> MNHKVHHHHHHIEGRVQALFNEISADAVFVTYDGQNIKKYGTHLDRAKTAYIPASTFKIANALIGLENHKATSTEIFKWDGKPRFFKAWDKDFTLGEAMQASTVPVYQELARRIGPSLMQSELQRIGYGNMQIGTEVDQFWLKGPLTITPIQEVKFVYDLAQGQLPFKPEVQQQVKEMLYVERRGENRLYAKSGWGMAVDPQVGWYVGFVEKADGQVVAFALNMQMKAGDDIALRKQLSLDVLDKLGVFHYL

OXA-58 is a carbapenem hydrolyzing class D β-lactamase (CHDL) expressed by the multi-drug resistant Acinetobacter baumannii. The enzyme hydrolyzes a variety of β-lactam antibiotics, including penicillins, cephalosporins, and the last resort carbapenems. Structurally, β-lactamase has a loop-rich region that includes the highly conserved Ω-loop. The Ω-loop of the class D β-lactamases contains a pivotal Trp residue that contributes to ζ-carbamic acid formation on the Lys base catalyst residue.

The crystal structure of OXA-58 showed the typical folding of a class D β-lactamase and consisted of six long β-strands and eight α-helices. The substrate-binding cleft between the two domains was a cavity in the loop-rich region that contained four loops: α3–α4 (97–122), Ω-loop (155–177), β6–β7 (225–230), and β8–α10 (254–260). Except for Ω-loop, the loops showed significantly different orientations from the previously reported structure and formed a narrower substrate-binding cleft. The cleft had an arch-like architecture formed by Phe113 and Phe114 of α3–α4, Met225 of β6–β7, and Ile260 of β8–α10, with the side chains of Phe113 and Met255 forming a roof over the cleft at a 4.2 Å distance. The Ω-loop was attached to a side end of the cleft through a short α-helix motif (Phe168–Trp169–Leu170–Lys171), and the indole ring of Trp169 in the Ω-loop was inserted into the active site. The side chain Νζ of Lys86 was carboxylated by NaHCO3 supplied during purification and crystallization. An oxygen atom of ζ-carbamic acid formed a bifurcated hydrogen bond with the nucleophile hydroxyl oxygen of Ser83 and the indole-NH nitrogen of Trp169 in the Ω-loop at distances of 2.6 Å and 2.9 Å, respectively. Thus, the hydrogen bond of the ζ-carbamic acid group and Trp169 formed a link between the active site and the Ω-loop. The loops α3–α4, β6–β7, and β8–α10 are flexible and mobile around the substrate-binding cleft as indicated by the up to 4-fold higher root-mean-square deviation (RMSD) compared with the overall average 0.49 Å RMSD. The averaged RMSD was 0.25 Å in the Ω-loop, which was significantly lower than the overall RMSD by 0.49 Å, thus indicating that the Ω-loop structure is static.> TEFKAGSAKKGATLFKTRCLQCHTVEKGGPHKVGPNLHGIFGRHSGQAEGYSYTDAAIKKNVLWDENNMSEY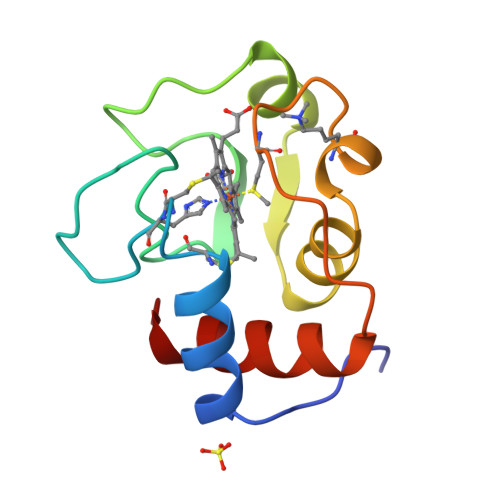LTNPKKYIPGTKMAFGGLKKEKDRNDLITYLKKATE> MASTGETTYKKTTSSALKGAIQLGITHSVG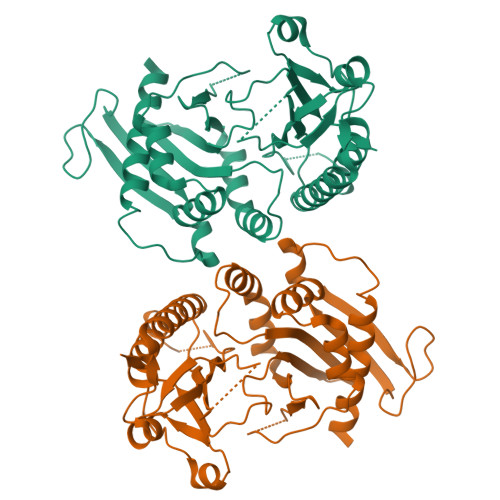SLSQKPERDVLMQDFEVVESIFFPSQGSSSTPGHHHGDFKFKTYAPIAFRYFREMFGIRPDDYLYSLCNEPLIELSNPGASGSLFYVSSDDEFIIKTVQHKEAEFLQTLLPGYFMNLNQNMRTLLPKFYGLYCVQADGKNIRIVVMNNLLPRAVPMHLKFDLKGSTYKRRASPKERSKGVPTYKDLDFMQDMPEGILLENDHYTALSRTMQRDCRVLQSFKIMDYSLLVGIHILHRAGEEASTAVPDTQKKGQGQKPLYCTAIESIQGESKSKTSPQPYESMGGIPAFNSKGERLLVFIGIIDILQSYRLVKKLEHSWKALLHDGDTVSVHRPSFYADRFQKFMCSTVFRKSQLKTLEHHHHHH> MVGLTTLFWLGAIGMLVGTLAFAWAGRDAGSGERRYYVTLVGISGIAAVAYAVMALGVGWVPVAERTVFVPRYIDWILTTPLIVYFLGLLAGLDSREFGIVITLNTVVMLAGFAGAMVPGIERYALFGMGAVAFIGLVYYLVGPMTESASQRSSGIKSL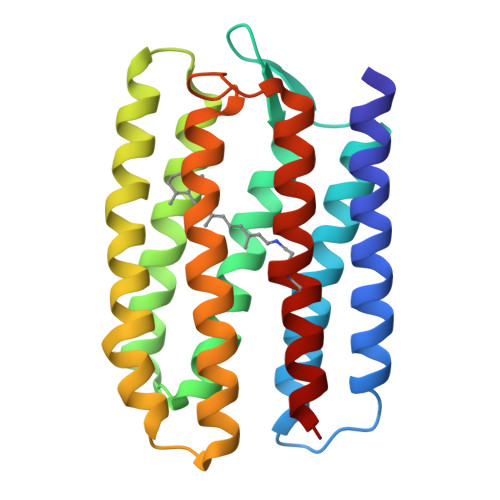YVRLRNLTVVLWAIYPFIWLLGPPGVALLTPTVDVALIVYLDLVTKVGFGFIALDAAA>[8x]MAHHHHHHSAALEVLFQGPGNNELSPVALRQMSCAAGTTQTACT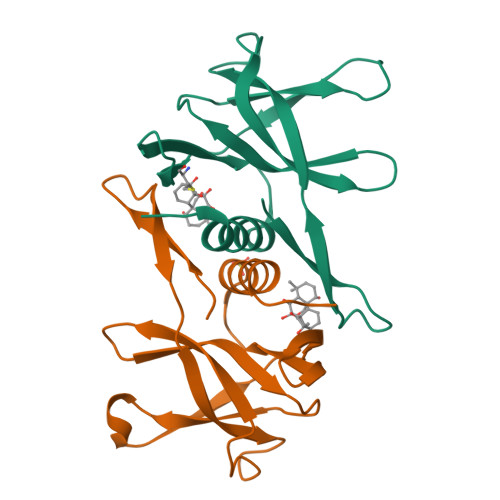DDNALAYYNTTKGGRFVLALLSDLQDLKWARFPKSDGTGTIYTELEPPCRFVTDTPKGPKVKYLYFIKGLNNLNRGMVLGSLAATVRLQ> DPVPQDASTKKLSECLKRIGDELDSNMELQRMI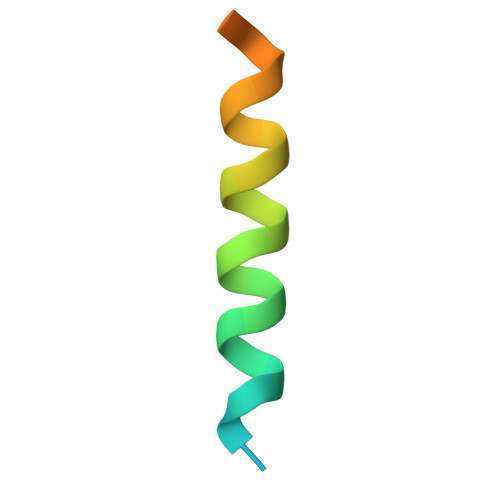A The GR is a ligand-regulated transcription factor (TF) that controls the expression of thousands of genes. GR has a domain structure common to the NR superfamily: an unstructured N-terminal domain, a zinc finger (ZnF)-containing DNA-binding domain (DBD), a hinge region and a ligand-binding domain. To modulate transcription, GR binds directly to DNA at canonical GBSs composed of two pseudo-palindromic hexameric repeats separated by a 3-bp spacer (5′-AGAACAnnnTGTTCT-3′). GR binds a canonical GBS as a dimer oriented in a head-to-head fashion.

Next, we biochemically characterize the extant human GR (hereafter GR, unless labeled otherwise) DBD bound to an unmethylated CpG-containing GBS (pre-GBS) and its methylated counterpart (5mC-GBS) and find that GR has preference for the 5mCpG GBS over the pre-GBS. Binding to the 5mC-GBS and pre-GBS showed Kd values of 131 and 206 nM, respectively. To determine how GR recognizes the 5mC-GBS and pre-GBS, we solved crystal structures of the GR DBD–5mC-GBS and GR DBD–pre-GBS complexes at a resolution of 2.0 and 2.5 Å, respectively. Both complexes crystallized in the C 1 2 1 space group and each structure contains a dimer of DBD protein molecules in the asymmetric unit. Crystal structures of these complexes reveal a specific van der Waals interaction between Arg447 in GR DBD and the methyl moiety in 5mC-GBS sequences, which is absent in the GR DBD–pre-GBS complex structure. We found that in the 5mC-GBS structure, Arg447 makes side-on hydrophobic contacts with the methyl group of the 5mC, mimicking interactions with a thymine base seen in extant GBSs. Without this interaction, Arg447 in monomer B moves outward but still makes hydrogen bonds with the guanine in CpG dinucleotide by one amide group, suggesting the methyl-derived side-on contact helps stabilize the Arg447. This gain of a hydrophobic contact could explain the increase in affinity from the unmodified pre-GBS to methylated pre-GBS. Each GR DBD monomer contacts the methylated pre-GBS with one more van der Waals contact than with an unmethylated pre-GBS, which results in larger buried solvent accessible surface area (BASA) between GR DBD and nucleotides in each half-palindromic site (140 Å2 versus 109 Å2 and 125 Å2 versus 115 Å2). We show that GR utilizes a similar methyl–Arg–G triad, suggesting that evolution has leveraged a readily available side-on interaction with the Arg residue engaged in recognizing the G base edge in a CpG dinucleotide.

>PPKLCLVCSDEASGCHYGVLTCGSCKVFFKRAVEGQHNYLCAGRNDCIIDKIRRKNCPACRYRKCLQAGMNLEAR[2x]>[4x]MSSSAMPDVPAPLTNLQFKYTKIFINNEWHSSVSGKKFPVFNPATEEKLCEVEEGDKEDVDKAVKAARQAFQIGSPWRTMD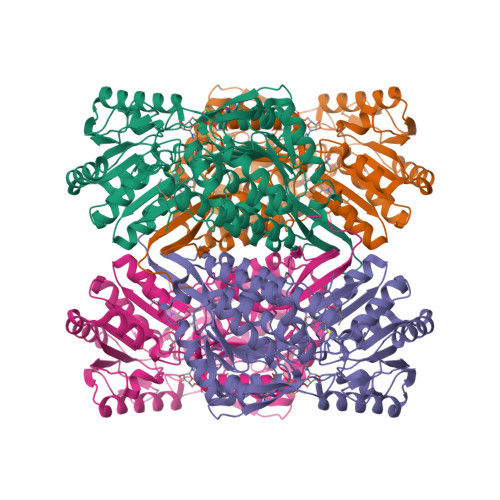ASERGRLLNKLADLIERDRLLLATMEAMNGGKLFSNAYLMDLGGCIKTLRYCAGWADKIQGRTIPMDGNFFTYTRSEPVGVCGQIIPWNFPLLMFLWKIGPALSCGNTVVVKPAEQTPLTALHMGSLIKEAGFPPGVVNIVPGYGPTAGAAISSHMDVDKVAFTGSTEVGKLIKEAAGKSNLKRVSLELGGKSPCIVFADADLDNAVEFAHQGVFYHQGQCCIAASRLFVEESIYDEFVRRSVERAKKYVLGNPLTPGVSQGPQIDKEQYEKILDLIESGKKEGAKLECGGGPWGNKGYFIQPTVFSDVTDDMRIAKEEIFGPVQQIMKFKSLDDVIKRANNTFYGLSAGIFTNDIDKAITVSSALQSGTVWVNCYSVVSAQCPFGGFKMSGNGRELGEYGFHEYTEVKTVTIKISQKNS>MSLQGIHLSDLSYKHAILKESQYTIKRDVGTTTAVTPSSLQQEITLLCGEILYAKHADYKYAAEIGIQYISTALGSERVQQILRNSGSEVQVVLTRTYSLGKIKNNKGEDLQMLDIHGVEKSWVEEIDKEARKTMATLLKESSGNIPQNQRPSAPDTPIILLCVGALIFTKLASTIEVGLETTVRRANRVLSDALKRYPRMDIPKIARSFYDLFEQKVYHRSLFIEYGKALGSSSTGSKAESLFVNIFMQAYGAGQTMLRWGVIARSSNNIMLGHVSVQAELKQVTEVYDLVREMGPESGLLHLRQSPKAGLLSLANCPNFASVVLGNASGLGIIGMYRGRVPNTELFSAAESYAKSLKESNKINFSSLGLTDEEKEAAEHFLNVSDDSQNDYE[2x];>[2x]MSFPEGKDILFMGNEAAKLAEAFQKSLRKPGHKRSQSIIGKHHHHHH

HMPV (Paramyxoviridae, subfamily Pneumovirinae) is a leading cause of serious respiratory tract infections in children, the elderly, and immunocompromised individuals. In all members of the Mononegavirales, the RNA genome is packaged in the form of a nucleocapsid, a ribonucleoprotein complex consisting of polymerized viral nucleoproteins (N) and RNA. Besides protecting the viral genome from host nucleases, the nucleocapsid serves as the template for transcription by the viral RNA-dependent RNA polymerase L. Nucleocapsid assembly necessitates a pool of monomeric, RNA-free N, termed N0, which is kept in an unassembled state through an interaction with an N-terminal portion of the polymerase cofactor P, until delivered to the sites of viral RNA synthesis. In conclusion, the reported structures of a paramyxoviral N protein reveal two distinct conformational states, N bound either to the polymerase cofactor P or to RNA.

To stabilize monomeric full-length N0 we fused the N-terminal domain of P to N, a strategy that has seen success with nucleoproteins from other viruses. We obtained crystals of RNA-free HMPV N in a monomeric state and bound to a P peptide at 1.9 Å resolution by adding trace amounts of trypsin to prune flexible loops and promote crystallization. In the structure, the P peptide is firmly nestled into a hydrophobic surface of the C-terminal domain of N (CTD) primarily composed of α-helices αC1 and αC2. Ile9, Leu10 and Phe11 of P occupy key positions and insert into this hydrophobic groove. The P peptide wraps around the CTD and residues 12–28 form an alpha helix that lies atop N. This helix is initiated at Gly12 and pinned to the CTD through an aromatic side-to-face interaction of Phe23 with Tyr354 of N, both residues belonging to the so-called mir motif which is conserved within Pneumovirinae. We observed that the binding site of the P peptide overlaps with the binding sites of the NTD- and CTD-arms. The downward, monomeric conformation is stabilized by specific salt-bridges linking the CTD-arm with the core of N. In this position the negatively charged CTD-arm folds into the positively charged RNA binding cleft, occupying it and directly blocking the binding of RNA. In the RNA-free state, Arg260 and Trp261 contact Glu375, while Arg186 forms a salt-bridge with Asp373 of the CTD-arm.>SMTPYEDLLRFVLETGTPKSDRTGTGTRSLFGQQMRYDLSAGFPLLTTKKVHFKSVAYELLWFLRGDSNIGWLHEHGVTIWDEWASDTGELGPIYGVQWRSWPAPSGEHIDQISAALDLLRTDPDSRRIIVSAWNVGEIERMALPPCHAFFQFYVADGRLSCQLYQRSADLFLGVPFNIASY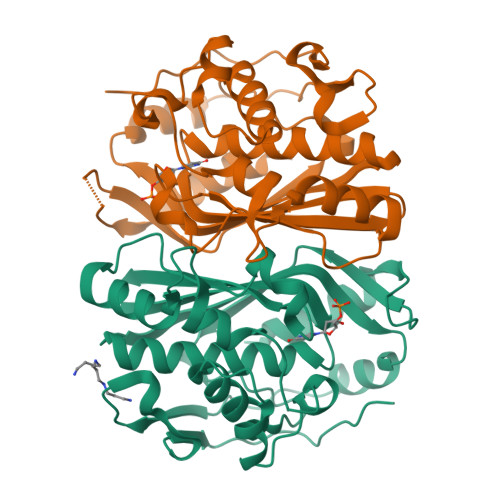ALLTHMMAAQAGLSVGEFIWTGGDCHIYDNHVEQVRLQLSREPRPYPKLLLADRDSIFEYTYEDIVVKNYDPHPAIKAPVAV[4x]> MFYALYFEIHHLVASAALGFARVAPIFFFLPFLNSGVLSGAPRNAIIILVALGVWPHALNEAPPFLSVAMIPL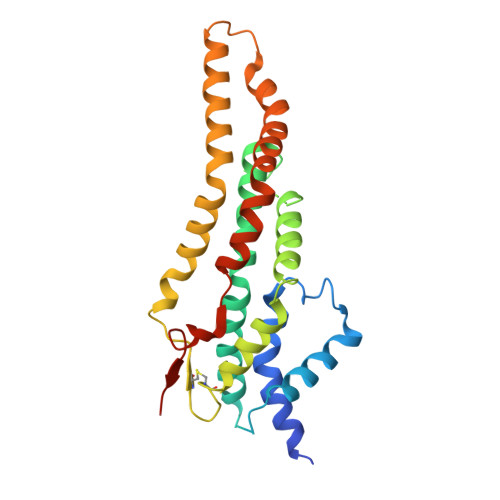VLQEAAVGVMLGCLLSWPFWVMHALGCIIDNQRGATLSSSIDPANGIDTSEMANFLNMFAAVVYLQNGGLVTMVDVLNKSYQLCDPMNECTPSLPPLLTFINQVAQNALVLASPVVLVLLLSEVFLGLLSRFAPQMNAFAISLTVKSGIAVLIMLLYFSPVLPDNVLRLSFQATGLSSWFYERGATHVLE> MKILKTLTLRGPNYWSIRRKKLIVMRLDLEDLAERPSNSIPGFYEGLIKVLPSLVEHFCSPGYQGGFLERVKEGTYMGHIVEHVALELQELVGMTAGFGRTRETSTPGVYNVVYEYVDEQAGRYAGRAAVRLCRSLVDTGDYPRLELEKDLEDLRDLGANSALGPSTETIVTEAEARKIPWMLLSARAMVQLGYGVYQQRIQATLSSHSGILGVELACDKEGTKTILQDAGIPVPRGTTIQYFDDLEEAINDVGGYPVVIKPLDGNHGRGITINVRHWQEAIAAYDLAAEESKSRAIIVERYYEGSDHRVLVVNGKLVAVAERIPAHVTGDGSSTISELIEKTNQDPNRGDGHDNILTKIVVNKTAIDVMERQGYNLDSVLPKDEVVYLRATANLSTGGIAIDRTDDIHPENIWLMERVAKVIGLDIAGIDVVTSDISKPLRETNGVIVEVNAAPGFRMHVAPSQGLPRNVAAPVLDMLFPPGTPSRIPILAVTGTNGKTTTTRLLAHIYRQTGKTVGYTSTDAIYINEYCVEKGDNTGPQSAGVILRDPTVEVAVLETARGGILRAGLAFDSCDVGVVLNVAADHLGLGDIDTIEQMAKVKSVIAEVVDPSGYAVLNADDPLVAAMADKVKAKVAYFS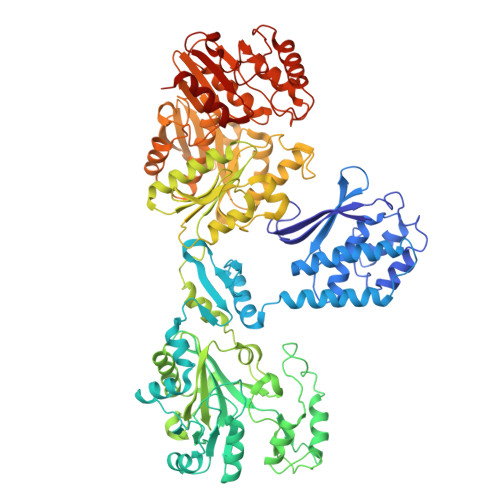MNPDNPIIQAHVRRNGIAAVYESGYLSILEGSWTLRVEQAKLIPMTMGGMAPFMIANALAACLAAFVNGLDVEVIRQGVRTFTTSAEQTPGRMNLFNLGQHHALVDYAHNPAGYRAVGDFVKNWQGQRFGVVGGPGDRRDSDLIELGQIAAQVFDRIIVKEDDDKRGRSEGETADLIVKGILQENPGASYEVILDETIALNKALDQVEEKGLVVVFPESVTRAIDLIKVRNPIGENLYFQ> QDADKLPHTKVT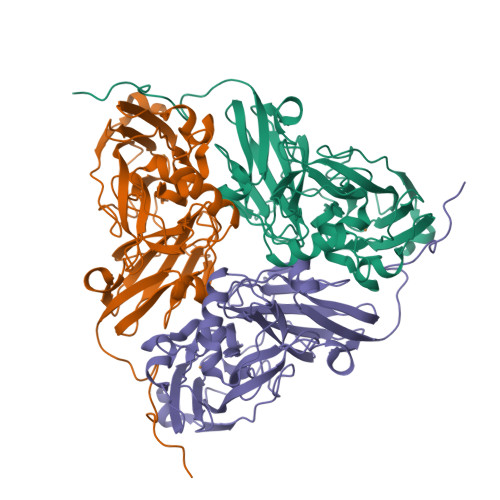LVAPPQVHPHEQATKSGPKVVEFTMTIEEKKMVIDDKGTTLQAMTFNGSMPGPTLVVHEGDYVQLTLVNPATNAMPHNVDFHGATGALGGAKLTNVNPGEQATLRFKADRSGTFVYHCAPEGMVPWHVVSGMSGTLMVLPRDGLKDPQGKPLHYDRAYTIGEFDLYIPKGPDGKYKDYATLAESYGDTVQVMRTLTPSHIVFNGKVGALTGANALTAKVGETVLLIHSQANRDTRPHLIGGFGDWVWETGKFANPPQRDLETWFIRGGSAGAALYTFKQPGVYAYLNHNLIEAFELGAAGHIKVEGKWNDDLMKQIKAPAPIPR The secretins are a large and diverse family of integral outer membrane (OM) proteins which comprise key components of the type II and type III secretion systems, as well as the biogenesis systems for type IV pili and filamentous bacteriophage. Our previous work on PilQ from Neisseria meningitidis showed a dodecameric structure, with a chamber sealed at both ends. Other proteins seem to play a more direct structural role: PilP is a lipoprotein which binds to PilQ and is essential for type IV pilus (TFP) formation. PilP thus forms a link between the OM, through its interaction with PilQ, and the inner membrane components of the type pilus biogenesis system.

In order to generate a structure which would allow docking of the domain structures presented above, we determined a 3D reconstruction of the complete PilQ dodecamer by cryoelectron microscopy. The final structure, measuring 155 Å in height and 110 Å at its widest external extent, forms a shell around a large internal chamber. The chamber is sealed at both ends, and a cut-away view shows evidence for distinct and separate structures within the density map (marked on the right hand side of Figure 6A). Structures of the B2 domain (B2PilQ224–329) and N0/N1 double domain (N0N1PilQ343–545) were docked into the cryoelectron density map using MULTIFIT, a program which has been shown to work well for structures with multiple components, even with low resolution maps. A striking feature of the resulting assembly is the location of the C-terminal helix in the N1 domain, which is orientated vertically, lining the sides of the top of the chamber and presumably forming a link to the transmembrane domain at the C-terminus. We therefore propose that the first β-domain adopts a partially folded structure in the PilQ oligomer, sufficient to contribute some density to the map, but have omitted it from our model as it remains poorly defined at present. PilP projects outward from the assembled PilQ complex, in an orientation which is different from the T2SS GspD-GspC complex: in that case, GspC was placed closer towards the interior of the secretin chamber. It is also readily apparent that the PilP C-terminal domain lies close to the B2 domain, essentially sandwiched as a ‘wedge’ between the N0 and B2 domains. One obvious function of PilP, therefore, is to stabilize the PilQ oligomer during secretion, preventing disassociation and consequent disruption of the channel.

>[12x]GNITDIKVSSLPNKQKIVKVSFDKEIVNPTGFVTSSPARIALDFEQTGISMDQQVLEYADPLLSKISAAQNSSRARLVLNLNKPGQYNTEVRGNKVWIFINESDDTVSAPARPAVKAAPAAPAKQQAAAPSTKSAVSVSEPFTPAKQQAAAPFTESVVSVSAPFSPAKQQAAASAKQQAAAPAKQQAAAPAKQQAAAPAKQTNIDFRKDGKNAGIIELAALGFAGQPDISQQHDHIIVTLKNHTLPTTLQRSLDVADFKTPVQKVTLKRLNNDTQLIITTAGNWELVNKSAAPGYFTFQVLPKKQNLESGGVNNAPKTFTGRKISLDFQDVEIRTILQILAKESGMNIVASDSVNGKMTLSLKDVPWDQALDLVMQARNLDMRQQGNIVNIAPRDELLAKDKAFLQAEKDIADLGALYSQNFQLKYKNVEEFRSILRLDNADTTGNRNTLISGRGSVLIDPATNTLIVTDTRSVIEKFRKLIDELDVPAQQVMIEARIVEAADGFSRDLGVKFGATGKKKLKNDTSAFGWGVNSGFGGDDKWGAETKINLPITAAANSISLVRAISSGALNLELSASESLSKTKTLANPRVLTQNRKEAKIESGYEIPFTVTSIANGGSSTNTELKKAVLGLTVTPNITPDGQIIMTVKINKDSPAQCASGNQTILCISTKNLNTQAMVENGGTLIVGGIYEEDNGNTLTKVPLLGDIPVIGNLFKTRGKKTDRRELLIFITPRIMGTAGNSLRY;>[12x]MKHYALLISFLALSACSQGSEDLNEWMAQTRREAKAEIIPFQAPTLPVAPVYSPPQLTGPNAFDFRRMETDKKGENAPDTKRIKETLEKFSLENMRYVGILKSGQKVSGFIEAEGYVYTVGVGNYLGQNYGRIESITDDSIVLNELIEDSTGNWVSRKAELLLNSSDKNTEQAAAPAAEQN> MRRSSSCLYKIPKNTGVAPRFDTWNEKYEPWEHLKRMGRLAGTGFYIPPEWYNHFRMFPPINHNFQQE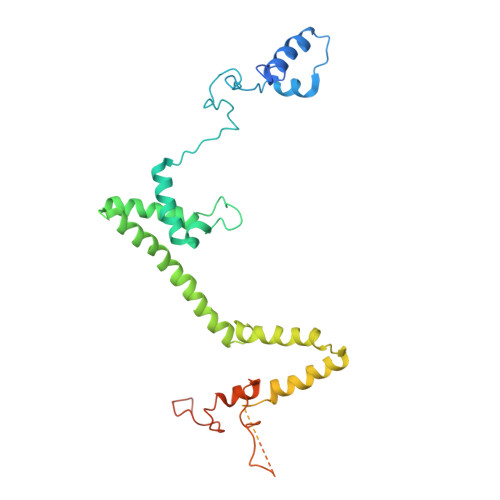KTLNPHNVSEPTQDDTDYLSVERIALRDELARKSRLLASEGMRYYNVFWIRKPLDRMERHYYELERKGVAHSVAIKRVLQMFYDELTVKKRVAAIQAEEAKLSGKYISMREATVLMGVLTQLQKEQLTPHQVTLLAKEQREKAQAGEAFAATVERSTETVADAAKDAAEGDEVMSADSLAELLSTEADLDDSSPSISYKVTIHETEHDSVKQLQELALDHTGKSDWYTGASPVLHMEEAMPAKRTPASKKTES>MKDVSKNQEENISDTALTNELIHLLGHSRHDWMNKLQLIKGNLSLQKYDRVFEMIEEMVIDAKHESKLSNLKTPHLAFDFLTFNWKTHYMTLEYEVLGEIKDLSAYDQKLAKLMRKLFHLFDQAVSRESENHLTVSLQTDHPDRQLILYLDFHGAFADPSAFDDIRQNGYEDVDIMRFEITSHECLIEIGLD[4x];>MMNEKILIVDDQSGIRILLNEVFNKEGYQTFQAANGLQALDIVTKERPDLVLLDMKIPGMDGIEIL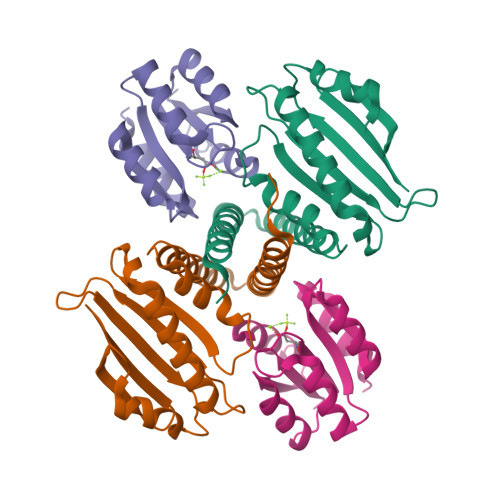KRMKVIDENIRVIIMTAYGELDMIQESKELGALTHFAKPFDIDEIRDAVKKYLPLKSN[4x]> MRRLAFLVVAFCLAVGCFFSPVSKAEGVMSGGDGDKVAVGKDGMVATAHPLASKIGAEVLKKGGNAIDAAIAIQYALNVTEPMMSGIG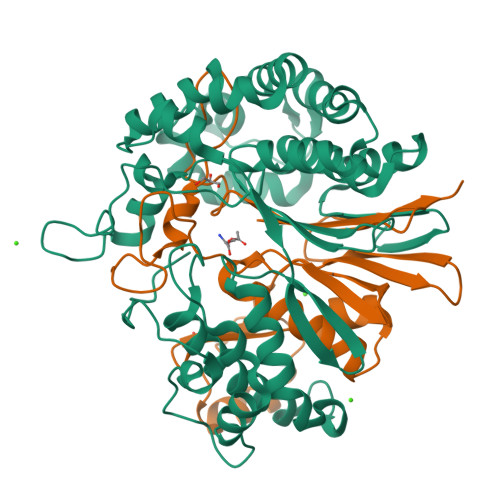GGGFMMVYDGETRETSIINSRERAPEGAKPDMFLDEDGKVIPFSERSRHGNAVGVPGTLKGLEAAHKKWGTKKMEDLISPSIKLTEEGFPIDSVLADAIKDHQDKLSKTAAKDIFLPDGEPLKEGDILVQKDLAKTFKLIRKEGSKAFYDGEIGRAIADVVQDFGGSMTPDDLSRYEVTTDKPIWGEYHGYDIASMPPPSSGGVFMLQVLKLIDDFHLSQYDPKSFEKYHLLAETMHLSYADRAAYAGDPEFVDVPLRGLLDPDYIKERQKLISLDSMNRDVKEGDPWKYEEGEPNYEIVPQPEDKTIGE;> TTHFTVTDQWGNVVSYTTTIEQLFGTGILVPGYGLFLNNELTDFDAIPGGANEVQPNKRPLSSMTPTIVFKDEKPVLTVGSPGGTTIIASVFQTILNYFEYGMSLQDAIEEPRIYTNSLTSYRYESGMPEDVRRKLNDFGHKFGSNPVDIGNVQSIFIDRENKTFMGVADSSRNGTAVGVNNKTSAE> MSLAKILVIDDESTILQNIKFLLEIDGNEVLTASSSTEGLRIFTENCNSIDVVITDMKMPKLSGMDILREI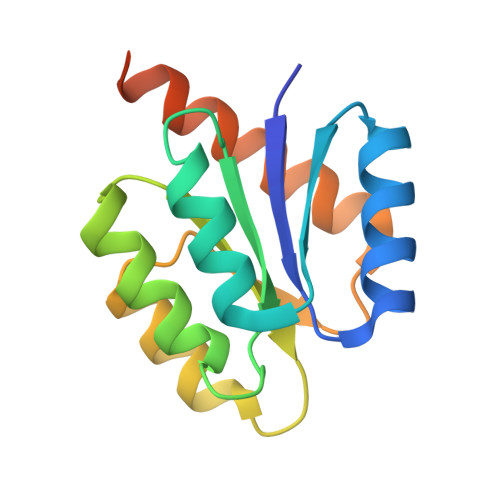KKITPHMAVIILTGHGDLDNAILAMKEGAFEYLRKPVTAQDLSIAINNAINRKKLLMENERMTQEGHHHHHH> GPLGSMLTLPEYNEQIPNVRSLLTKWAKVERIQDVQDGLQLDVRLKTDTLLELHIYYDHVYHVPSIKFRLWSLDTEEDISSLRLLTLSDSELRSILNLGTFSVTLSTDMEMKSVYYYINNCDTDANVGSDVEHYLTRWISLY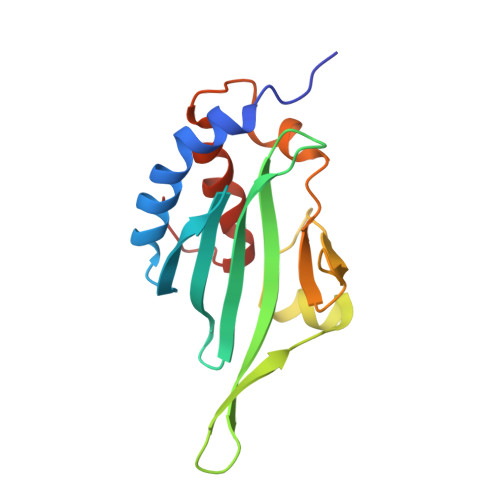IRIFDLNFVP>[2x]DCHLSDMLQQLHSVNASKPSERGLVRQEEAEDPACIPIFWVSKWVDYSDKYGLGYQLCDNSVGVLFNDSTRLILYNDGDSLQYIERDGTESYLTVS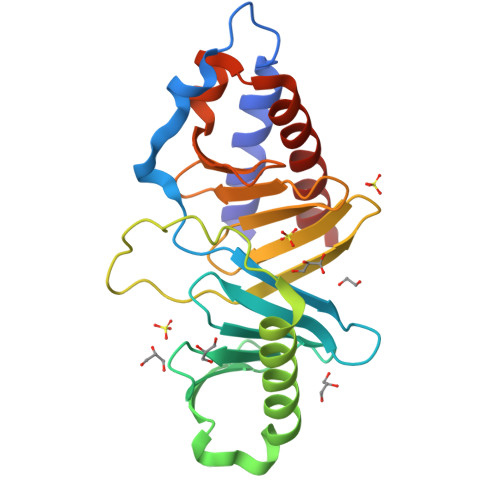SHPNSLMKKITLLKYFRNYMSEHLLKAGANITPREGDELARLPYLRTWFRTRSAIILHLSNGSVQINFFQDHTKLILCPLMAAVTYIDEKRDFRTYRLSLLEEYGCCKELASRLRYARTMVDKLLSS> GPLGSWSWESYLEEQKAITAPVSLFQDSQAVTHNKNGFKLGMKLEGIDPQHPSMYFILTVAEVCGYRLRLHFDGYSECHDFW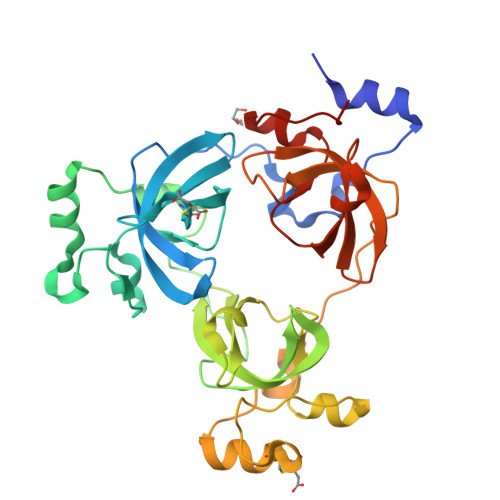VNANSPDIHPAGWFEKTGHKLQPPKGYKEEEFSWSQYLRSTRAQAAPKHLFVSQSHSPPPLGFQVGMKLEAVNRMNPSLVCVASVTDVVDSRFLVHFDNWDDTYDYWCDPSSPYIHPVGWCQKQGKPLTPPQDYPDPDNFCWEKYLEETGASAVPTWAFKVRPPHSFLVNMKLEAVDRRNPALIRVASVEDVEDHRIKIHFDGWSHGYDFWIDADHPDIHPAGWCSKTGHPLQPPLG> RPNHTIYINNLNEKIKKDELKKSLHAIFSRFGQILDILVSRSLKMRGQAFVIFK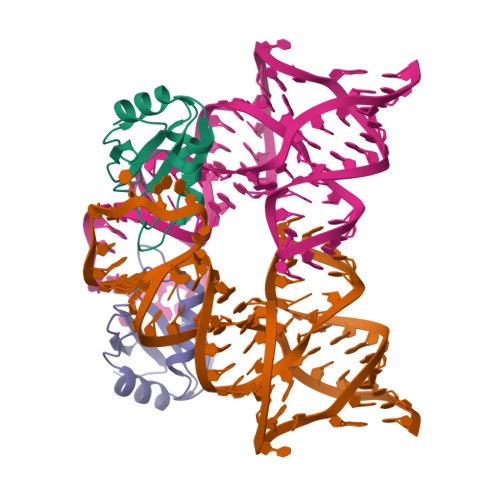EVSSATNALRSMQGFPFYDKPMRIQYAKTDSDIIAKM> SNAMAGHSKWANIKHAKARQDAKRGKVFTKLIREITVAARLGGEDIDSNPRLRAVVDKAFAANMPKDTITRAIKRGAGSGAGDNLVEVRYEGYGPSGVAVMVDCLTDNKNRTVAEVRHAFSKCDGNLGTEGSVAYLFKQRGLITFPPNSDEEKIMEIALEVGAEDVTTNDDGSIDVTTLPEDFEKIRNAMKAADLNPSHAEVTVLASTEVGLDKDSAEQMLRLTEMLEDLD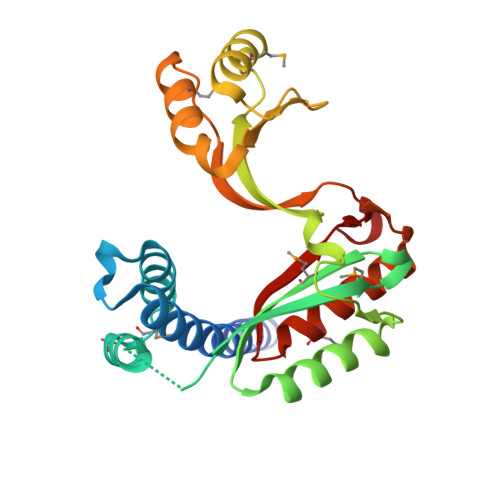DVQNVYSNADYPEEVL>[2x]RRYTLNATALGLGGAATRQLTFQTSSPAHLTMPYVMPGDGEV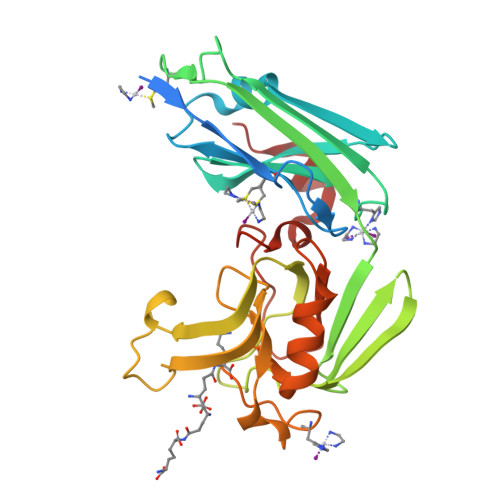VGVGEPVAIRFDENIADRGAAEKAIKITTNPPVEGAFYWLNNREVRWRPEHFWKPGTAVDVAVNTYGVDLGEGMFGEDNVQTHFTIGDEVIATADDNTKILTVRVNGEVVKSMPTSMGKDSTPTANGIYIVGSRYKHIIMDSSTYGVPVNSPNGYRTDVDWATQISYSGVFVHSAPWSVGAQGHTNTSHGCLNVSPSNAQWFYDHVKRGDIVEVVNTVGGTLPGIDGLGDWNIPWDQWRAGNAKA> 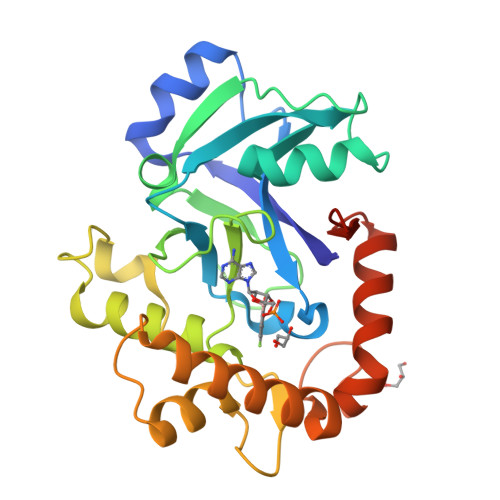MGYVGIKIRLTDVAPQAQELFKKESLDVKENKVYLVAATLRPETMYGQTCCFVSPKIDYGVFDAGNGDYFITTERAFKNMSFQNLTPKRGYYKPLFTINGKTLIGSRIDAPYAVNKNLRVLPMETVLATKGTGVVTCVPSDSPDDFVTTRDLANKPEYYGIEKDWVQTDIVPIVHTEKYGDKCAEFLVNDLKIQSPKDSVQLANAKELAYKEGFYNGTMLIGKYKGDKVEDAAPKVKQDLIDEGLAFVYNEPELEHHHHHH>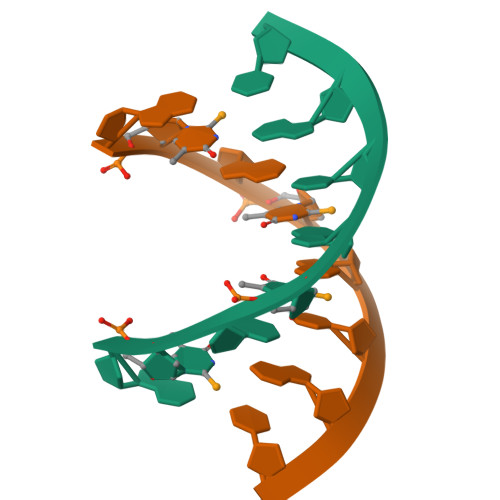[2x]GTGTACAC> MAKRRNRKTRFNLPPGKSGWPFLGETIGYLKPYTATTLGDFMQQHVSKYGKIYRSNLFGEPTI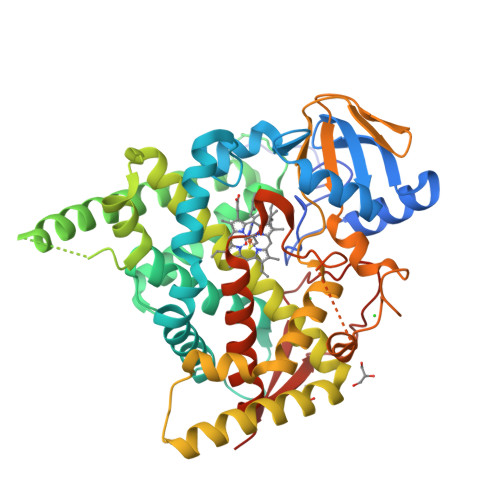VSADAGLNRFILQNEGRLFECSYPRSIGGILGKWSMLVLVGDMHRDMRSISLNFLSHARLRTILLKDVERHTLFVLDSWQQNSIFSAQDEAKKFTFNLMAKHIMSMDPGEEETEQLKKEYVTFMKGVVSAPLNLPGTAYHKALQSRATILKFIERKMEERKLDIKEEDQEEEEVKTEDEAEMSKSDHVRKQRTDDDLLGWVLKHSNLSTEQILDLILSLLFAGHETSSVAIALAIFFLQACPKAVEELREEHLEIARAKKELGESELNWDDYKKMDFTQCVINETLRLGNVVRFLHRKALKDVRYKGYDIPSGWKVLPVISAVHLDNSRYDQPNLFNPWRWQQQNNGASSSGSGSFSTWGNNYMPFGGGPRLCAGSELAKLEMAVFIHHLVLKFNWELAEDDKPFAFPFVDFPNGLLIRVSRILHHHH4-[(2S,3R)-3-[3,5-bis(oxidanylidene)piperazin-1-ium-1-yl]butan-2-yl]piperazin-4-ium-2,6-dione 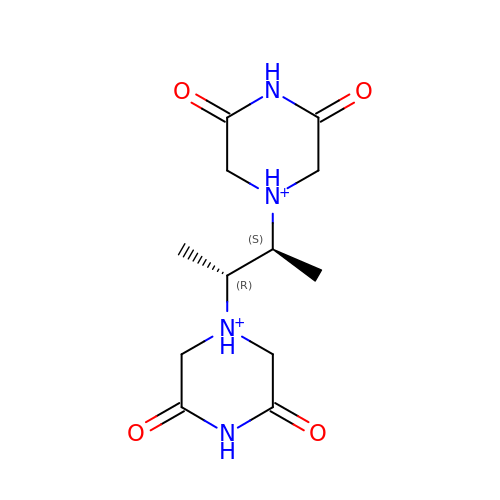| C12 H20 N4 O4 | OBYGAPWKTPDTAS-OCAPTIKFSA-P>[2x]DLSQCDREPIHLLGGIQSHGVLLAFRGPDRLLEVVSANAQALLGRPPETLLGQPVGRVLPAEVLAQWEPLVARGSVRVVLPAG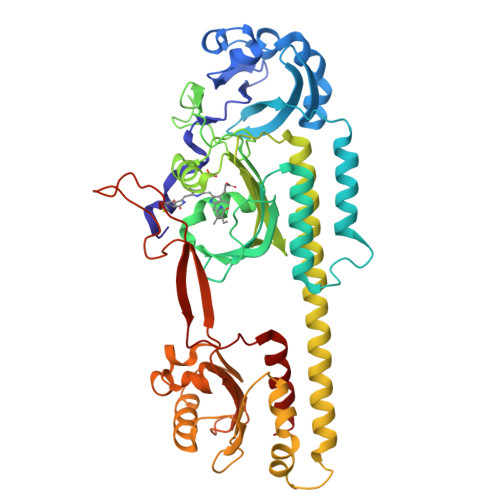AYRALLHESDGLTVLELEPAELQPGMEETALEVVRRLVSPLAGVKGTQALLQTAADTVRALTGFDRVMVYRFDADWHGEVLAESKRGGMDGFLGMHFPATDIPVQARALYTRNPLRLIADARARPVPLLPPVVPALGRPLDLSNSALRSVSPVHLEYLRNMGVGASFSLSLLKEGVLWGLIACHHLEPLHISHERRRACEVLTQLLALQLSAEERAAEASEDAHRAALLGQLATAMGEGGTLEEVLEKESERVLALTGAAGVALLLGEEPLLVGCTPAQDEVEALVAWLATQPFQTSFHTDRLGTVYPPLAARADVAAGILAVRLAPAAARFAIWFRPEVARTISWAGNPRKPAEPEPGHQRLHPRGSFQAWEETVRDTSLPWKRADLGAAEGFRGAL> MSVTGVFSKGRGIGHAAVTSILRYIPRARVPWQPSRFGRENLSASDLAVLWSRGRYRDGPGNYNSGYHTEKTHVLEDNTVTMIPKHELEKYMPDISIGPKALVTPVSLMSARNGHRVTHDLLHSYDPHIGRLDKPAVVDHDNITVEDPNRVGLNAATLDCRGRIYRWLRRGPFFQEDHYFRRSLRLNRDGTVPTAAHEAPLMRKIVRLAQRGHLKAACEEYRRVTTVPPVEVYRALTACCIPGGLIADAVAIFEDGNSKLFYVARDGEVLHNVMRCAIKAKNRVRVMWVYNVMRGRYYENVIVRAEIDPIWRYRIALLALEYFLDHNCAEEAGTVYSYLVEEDLLQCDVHLRVGLHMREALSKGKSVGLSDEVLRATSLVTDVATVAPEVARELYQRHVEALRENEKSNDCDMNTKNDGATGCAWSAHGLLTALDFTQKDDALPWMQQNFGDVDVASVLRWARFYHSKDLMAKDRPRYLARAVAWIELLSKRSHMMEEAPLTYMRKSKPLSLNTN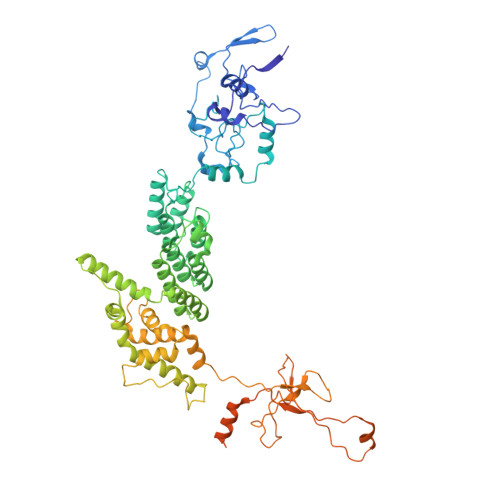SNLRVAWQTPVARPDGPPRLLAREEGYTFHHNEHSRFVTETYRHPGETLQSRFLAMQPIHTEVSAKEDFQEIYAQQQEQRALPSGVVSPTARILHHSVTSEIHGGGGGQHHRSMSRAESSTGGAVKKEKLNLVSPHVAAEKRGGSGTGNIGGTAAGGGVTPEF> MVANPPKPFEVHESGAYLHGTKAELKVGDRLVPGRESNFEAGRIMNHIYITQTLDAAVWGAELAAGEGRGRIFIVEPEGAIE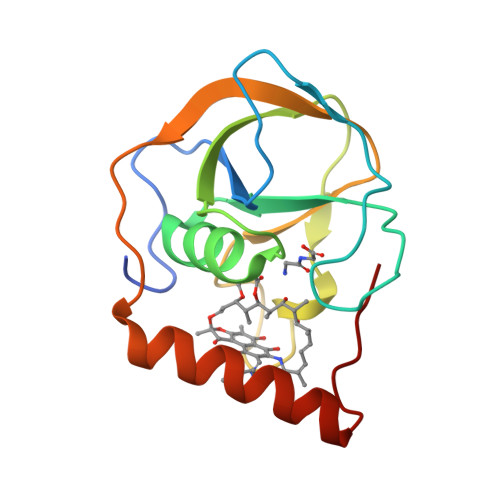DDPNVTDKKLPGNPTRSYRTREPVWIVGELTDWVGHPPEQLAAMRQGLEELRRKGLAVIYD4-({5-amino-1-[6-(2-cyanoethyl)naphthalene-1-sulfonyl]-1H-1,2,4-triazol-3-yl}amino)-2-chlorobenzonitrile | C22 H16 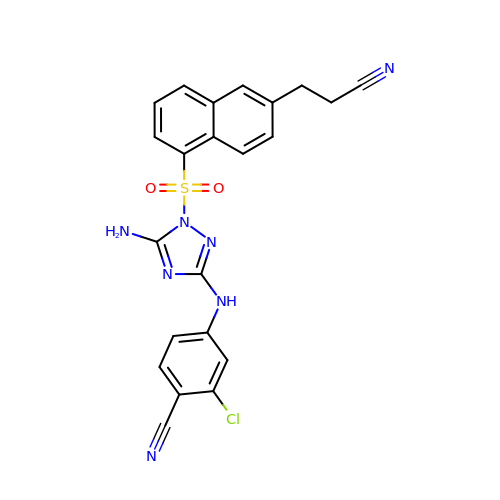Cl N7 O2 S | YLHDIFMTTOCZFP-UHFFFAOYSA-N>[2x]XSDIAFLIDGSGSIIPHDFRRMKEFVSTVMEQLKKSKTLFSLMQYSEEFRIHFTFKEFQNNPNPRSLVKPITQLLGRTHTATGIRKVVRELFNIT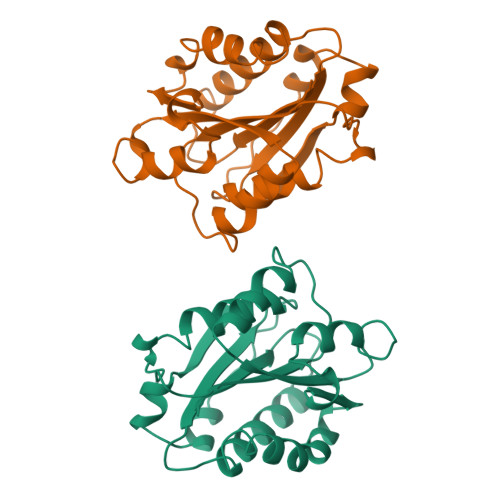NGARKNAFKILVVITDGEKFGDPLGYEDVIPEADREGVIRYVIGVGDAFRSEKSRQELNTIASKPPRDHVFQVNNFEALKTIQNQLREKIFAIEG> GSHMLRLSAPGQLDDDLCLLGDVQVPVFLLRLGEASWALVEGGISRDAELVWADLCRWVADPSQVHYWLITHKHYDHCGLLPYLCPRLPNVQVLASERTCQAWKSESAVRVVERLNRQLLRAEQRLPEACAWDALPVRAVADGEWLELGPRHRLQVIEAHGHSDDHVVFYDVRRRRLFCGDALGWFDEAEGVWRPLVFDDMEAYLESLERLQRLPTLLQLIPGHGGLLRGRLAADGAESAYTECLRLCRRLLWRQSMGESLDELSEELHRAWGGQSVDFLPGELHLGSMRRMLEILSRQALPLD

PqsE has two biochemical activities, a protein–protein interaction with RhlR, which increases RhlR transcriptional activity at target promoters, and an esterase activity. Curiously, RhlR function additionally depends on the metallo-β-hydrolase enzyme PqsE, encoded as the final gene in the pqsABCDE biosynthetic operon. With respect to RhlR, PqsE is required to form a protein–protein interaction that enhances the affinity of RhlR for target promoters. The effects of the PqsE E182W and PqsE NI substitutions on pyocyanin production are not through impairment of PqsE catalytic function, as the catalytically inactive variant, PqsE(D73A), remains fully capable of interacting with RhlR and driving pyocyanin production. These results indicate that PqsE has two independent functions, catalysis and interaction with RhlR, and it is interaction with RhlR, not catalysis, that is required for virulence. Moreover, the RhlR–PqsE interaction is essential for P. aeruginosa virulence phenotypes, and therefore, of interest as a focus for antibiotic development.

We recently showed that the ability of PqsE to interact with RhlR can be weakened by the introduction of an “inhibitor mimetic” mutation in which the glutamate residue at position 182 is altered to tryptophan [PqsE(E182W)].24 The PqsE(E182W) variant is a stable protein that, while harboring all of the catalytic residues, nonetheless displays less than 10% of wildtype catalytic activity, as if an inhibitor is bound in the active site. To understand, at an atomic level, what conformational changes the E182W alteration induced in PqsE to affect its ability to interact with RhlR, we determined the structure of PqsE(E182W). Although the PqsE(E182W) crystals grow in the same P3221 crystal form as WT PqsE, there is a significant structural rearrangement in the active site. In WT PqsE, the sidechain of E182 lies at the edge of the ligand binding site and makes hydrogen bonds with R191 and Q272. These interactions do not occur in PqsE(E182W), and rather, new interactions are made between the sidechain of the introduced W182 residue and F276, L277, and P278. The E182W change induces the rearrangement of the G270-L281 loop between helices 6 and 7, with a portion of that loop becoming disordered. Examination of electron density within the active site indicated a surprising consequence—with the sidechain of E280 relocating by 12 Å and becoming Fe bound in the center of the active site. Indeed, the repositioned E280 sidechain directly binds both Fe atoms, acting as a bridging ligand, and thus is most likely responsible for the stabilizing effect the E182W alteration has on PqsE, which we have reported previously. The crystal structure of PqsE(E182W) revealed that a loop rearrangement inserts the E280 residue into the active site to coordinate both of the iron atoms at this site.> NLSDVDLSKYITTIAGVMTLSQVKGFVRKNGVNEAKIDEIKNDNVQDTAEQKVQLLRNWHQLHGKKEAYDTLIKDLKKANLCTLAEKIQT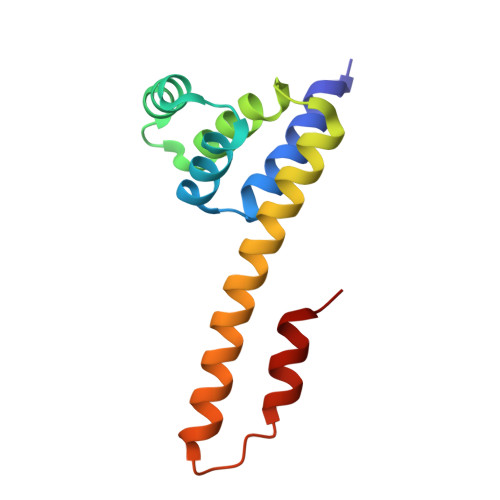IILKDITSDSENSNFRNEIQSLVLE> MYVYKRDGRKEPVQFDKITARISRLCYGLDPKHIDAVKVTQRIISGVYEGVTTIELDNLAAETCAYMTTVHPDYATLAARIAISNLHKQTTKQFSKVVEDLYRYVNAATGKPAPMISDDVYNIVMENKDKLNSAIVYDRDFQYSYFGFKTLERSYLLRINGQVAERPQHLIMRVALGIHGRDIEAALETYNLMSLKYFTHASPTLFNAGTPKPQMSSCFLVAMKEDSIEGIYDTLKECALISKTAGGIGLHI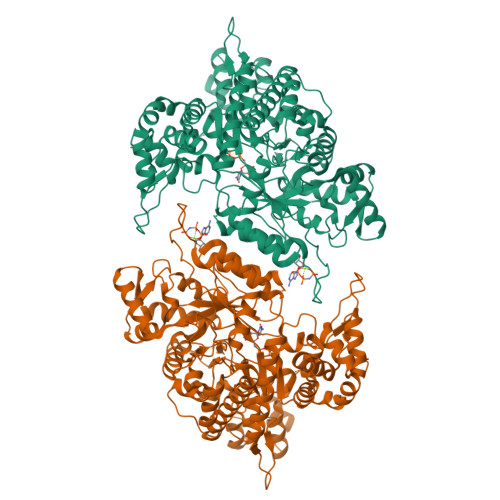HNIRSTGSYIAGTNGTSNGLIPMIRVFNNTARYVDAGGNKRPGAFALYLEPWHADIFDFIDIRKNHGKEEIRARDLFPALWIPDLFMKRVEENGTWTLFSPTSAPGLSDCYGDEFEALYTRYEKEGRGKTIKAQKLWYSILEAQTETGTPFVVYKDACNRKSNQKNLGVIKSSNLCCEIVEYSAPDETAVCNLASVALPAFIETSEDGKTSTYNFKKLHEIAKVVTRNLNRVIDRNYYPVEEARKSNMRHRPIALGVQGLADTFMLLRLPFDSEEARLLNIQIFETIYHASMEASCELAQKDGPYETFQGSPASQGILQFDMWDQKPYGMWDWDTLRKDIMKHGVRNSLTMAPMPTASTSQILGYNECFEPVTSNMYSRRVLSGEFQVVNPYLLRDLVDLGIWDEGMKQYLITQNGSIQGLPNVPQELKDLYKTVWEISQKTIINMAADRSVYIDQSHSLNLFLRAPTMGKLTSMHFYGWKKGLKTGMYYLRTQAASAAIQFTIDQKIADQATENVADISNLKRPSYMPSSASYAASDFVPAAVTANATIPSLDSSSEASREASPAPTGSHSLTKGMAELNVQESKVEVPEVPAPTKNEEKAAPIVDDEETEFDIYNSKVIACAIDNPEACEMCSG> MIWKYLQRTNRGNIIQAGLQHRKFENLPFKQNFDNLTKAYDLRMWYISNSPHEAKNLEYVNELEALHNELNYQNSRQFLFRTVSFLLGWALFYQFYELPKTYD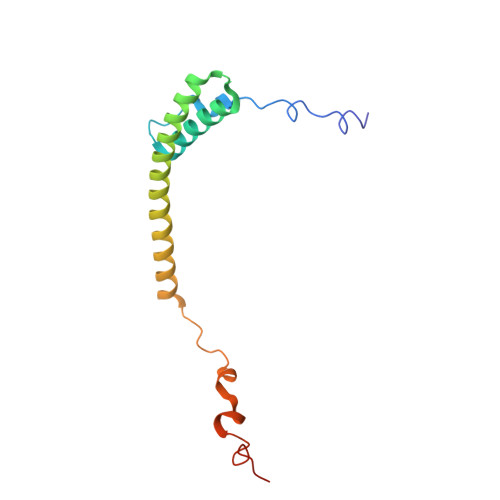WQDTQEPKHQVPAYGDLEEGGDEGGDD>[4x]VTYPGAIPLSLTSNYETPSPTAIPLEPTPTATGTAELDALWNLVEAQYPVQTAAVTTLVTVPDDYKFEADPPSYALAGYETSEIAGLKFPKGFKFGVAGAAIQVEGAAKAEGRGPSTWDYLCHHYASTQCNNYDPDITTNHYYLYPLDFARLQHLGINTYSFSISWTRIYPLGAGYVNEAGLAHYDAVIHSAKKYGLEPVGTVFHWDTPLSLMLKYGAWQDTGDQIVKDFVTYATTVFKRYGNEVKTWFTFNEPRVFCSQNSGLPYNLTYPEGINSTSAVFRCTYNVLKAHGHAVKVYRDLVASGTIAAGEIGFKSDDNYPIPARPGNADDEESAKRHEAFRIGIFAQPVYGNGDYPDVVKETVGDMLPALTDEDKGYIKGSGDIFAIDGYRTDISHAALNGIANCIRNQSDPNWPVCEEGSDPFAHVYPSGFAIGQSADPLSSWLVNSAPFIR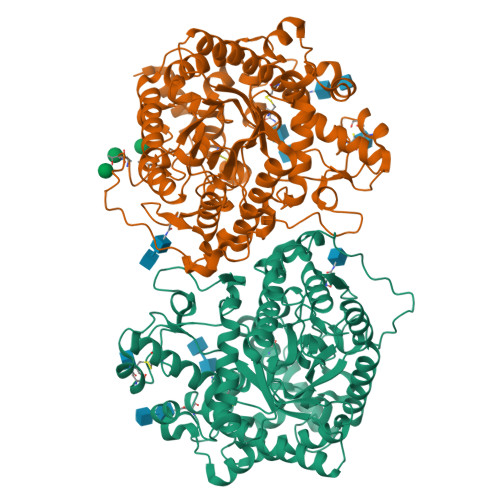DQLKFLTQTYPAKGGIYFSAFGWAEDAEYDRQLLYQITWDGLRTQYLTDYLSQLLLAVHKDGINLRGALTWSFVDNWEWGLGMQQKFGFQFVNQSDPDLTRTFKLSAHAYAQFGRNHLHHHHHH> MFPFALLYVLSVSFRKIFILQLVGLVLTYDFTNCDFEKIKAAYLSTISKDLITYMSGTKSTEFQNTV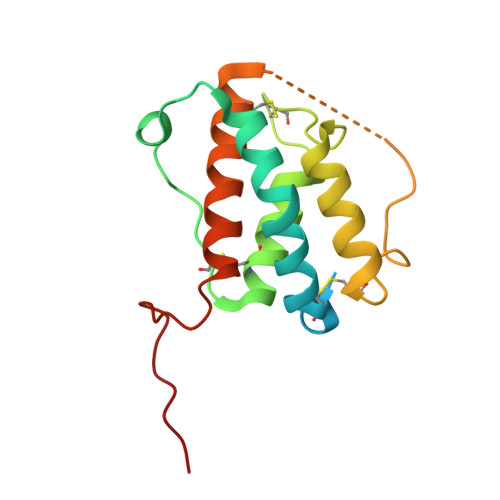SCSNRPHCLTEIQSLTFNPTAGCASLAKEMFAMKTKAALAIWCPGYSETQINATQAMKSVTTNKCLEQVSQLQGLWRRFNRPLLKQQGTKHHHHHH>[2x]MAHHHHHHSAARLMKLDWERTGRRMGFIDLSKYEVWSYDTECTGLQYKVDKVFGFSIATPDGQSGYFDVREQPESLQWLAEQVEPYKGTIVCHNASFDYRMSLHSGIKLPLSQIDDTGIRACCINEHESTIFPWTRGRAGDYSLDYLAKKYVGAQKYAEIYDELAALFGGKATRKTQMPNLYRAPSGLVRKYACPDAELTLELWLEQEELIKKRGLERIVAFERKVMPTLIRT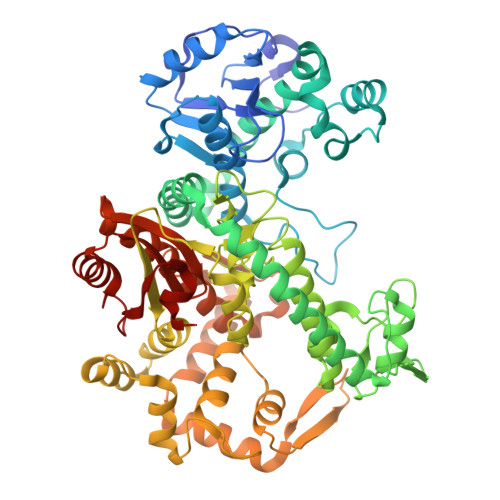EARGVRVDLDYAEQAIFKMDGVVRENQAKMFALAGREFNPNSPKQVREVFGAKEEGGVWKSRDGTILERTATGNPCLDADALRSMTDPLAAAVLELRSNIKTKDTFLAKHVVEHSVGGRVYPNINQMKGEDGGTGTGRLSYTGPALQQIPSRNKRIAAIIKPAFLPEEGQLWLDSDMASFEVRIFAHLVAAYNPAIAKAYAENPELDLHQWVGDLMGIPRNASYSGQPNAKQMNLGMIFNRGDGAVADSLGMPWEWCEFTDKKGELIRYKKAGREAKSIIAAYHSQIQGVKTLATRAQKIAEERGWIQTAHGRRLRFPNGYKSYKASGILIQATAADENKENWLRIEDALGSDGSMILNTHDSYSMSVDENWKPIWERVKKAVERQTLRVPLLLEFDGVGKNWAEAKGLIDVH> MLQKNTLLFAALSAALWGSATQAADAAVVASLKPLGFIASAIADGVTDTQVLLPDGASEHDYSLRPSDVKRLQGADLVVWVGPEMEAFMEKSVRNIPDNKQVTIAQLADVKPLLMKGAGEYNMHLWLSPEIARATAVAIHEKLVELMPQSRAKLDANLKDFEAQLAATDKQVGNELAPLKGKGYFVFHDAYGYYEKHYGLTPLGHFTVNPEIQPGAQRLHEIRTQLVEQKATCVFAEPQFRPAVVEAVARGTSVRMGTLDPL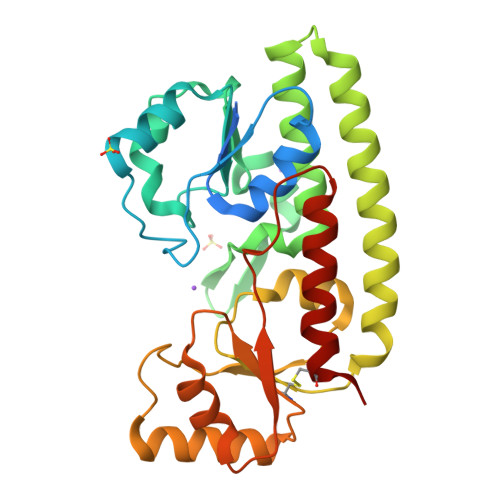GTNIKLGKTSYSAFLSQLANQYASCLKGD> MPVKVCLIFAGGTGMNVATKLVDLGEAVHCFDTCDKNVVDVHRSVNVTLTKGTRGAGGNRKVIL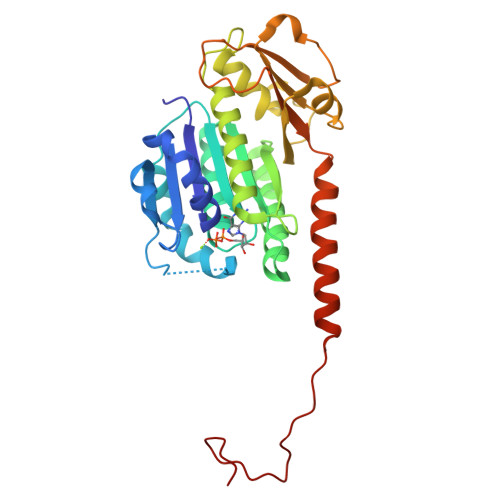PLVRPQIPALMDTIPEADFYIVCYSLGGGSGSVLGPLITGQLADRKASFVSFVVGAMESTDNLGNDIDTMKTLEAIAVNKHLPIVVNYVPNTQGRSYESINDEIAEKIRKVVLLVNQNHGRLDVHDVANWVRFTDKHNYLIPQVCELHIETTRKDAENVPEAISQLSLYLDPSKEVAFGTPIYRKVGIMKVDDLDVTDDQIHFVINSVGVVEIMKTITDSKLEMTRQQSKFTQRNPIIDADDNVDEDGMVV>[4x]MEAEEDGDLQCLCVKTTSQVRPRHITSLEVIKAGPHCPTAQLIATLKNGRK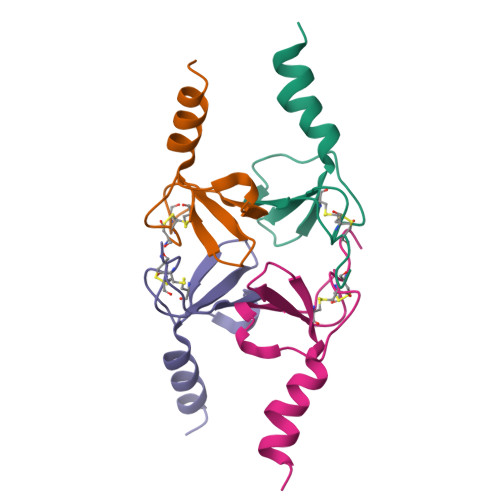ICLDLQALLYKKIIKEHLES>MVLYFIGLGLYDERDITVKGLEIAKKCDYVFAEFYTSLMAGTTLGRIQKLIGKEIRVLSREDVELNFENIVLPLAKENDVAFLTPGDPLVATTHAE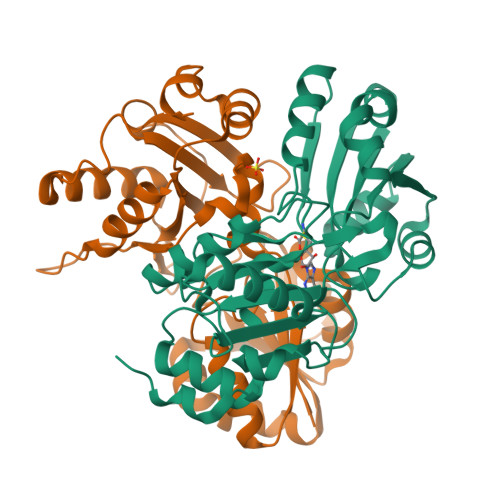LRIRAKRAGVESYVIHAPSIYSAVGITGMHIYKFGKSATVAYPEGNWFPTSYYDVIKENAERGLHTLLFLDIKAEKRMYMTANEAMELLLKVEDMKKGGVFTDDTLVVVLARAGSLNPTIRAGYVKDLIREDFGDPPHILIVPGKLHIVEAEYLVEIAGAPREILRVNV[2x]>MNPTIIRARAPLRLGLAGGGTDVAPYADTFGGYVLNATIDRYAYAVIKTLTIPAVRFVSTDQQVEKHQLISEPLELNGTLNLHKAVYNHMIRNYNHGKPIALELSTFCDAPAGSGLGSSSTLVVVMIKAFVELLNLPLDDYAIAQLAYRIERVDCGLAGGRQDQYSATFGGFNFMEFYAAARTIVNPLRIKNWVLCELEASLVLFYTGVSRESAKIIQDQSDNVVSHKTAAIEAMHGIKREALVMKEALLKGDFKAFVASMRLGWDNKKNSARTVSNAHIDEIYDAAIRAGAQAGKVSGAGGGGFMLFFVPTEKRMDLIRTLGEYDGQVSNCHFTKNGTQAWRIAN[2x]

Here, we present the structure of WcbL from Burkholderia pseudomallei. A critical step in the synthesis of heptoses is their 1-O phosphorylation, mediated by kinases such as HldE or WcbL. We report that WcbL operates through a sequential ordered Bi-Bi mechanism, loading the heptose first and then ATP. The protein forms a head-to-tail dimer, with the two active sites facing away from the dimer interface, in line with the native molecular weight predicted from size-exclusion chromatography.

Repeated attempts to soak or co-crystallize the substrates M7P and ATP failed. However, soaking with the non-hydrolyzable substrate analog AMP-PNP showed clear density for this nucleotide. The ATP analog appears to form a network of interactions with the enzyme, with the majority of interactions formed with the phosphate, and the ribose O2 and O3 hydroxyls. The phosphates interact with the side chains of R13 and D163, while the ribose ring interacts with the side chains of S118 and S119. The structure of WcbL bound to AMP-PNP suggests that the ATP may bind in a manner that blocks access to the sugar-phosphate binding site. Superimposing the locations of AMP-PNP and mannose shows that the location of these molecules is compatible. Indeed, the reactive atoms (O1 of mannose, Pγ of AMP-PNP) are located in positions compatible with the expected reaction (nucleophilic attack of O1 on the γ-phosphate). This suggests that the locations of these two substrate analogs in the structure are representative of the true ligands. Native WcbL and an AMP-PNP complex had a lower proportion of the monoclinic fraction: for these complexes data did not process well and the model did not refine in the monoclinic space group.>[6x]MNVQAHLFVSLGTAPAIVPEAFLLPGARFVSVHVLTTERPDVTLIREFFRRHAPGVNLTITRVAGFQDLKSEEDHFRFEEVMFRWFLASRTGPEQRFVCLTGGFKTMSAAMQKAATVLGAAEVFHVLADDCCVGPQGRLMPPSTLEEILWARDQGHLHWIRLGPERGWPQLRRIA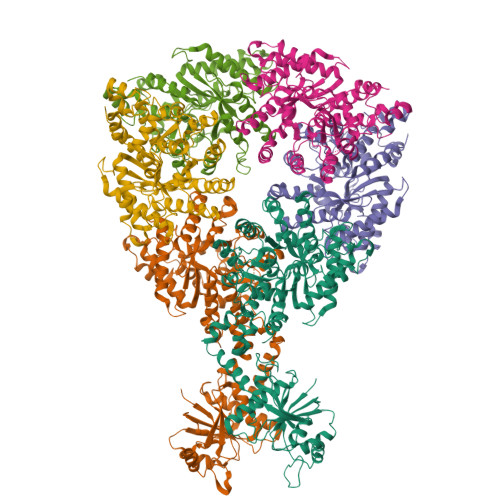PEQFPLQVVEEKGDERRVQAEDRAFGTFLQDLLQRASRIAGAWEMLPELPFADLATWSEGELAWLREPLDPRAPADQRWVAGLPKIELHCHLGGFATHGELLRRVRNAAENPGKLPPLEEPRLPEGWPLPAQPIPLAEYMKLGNANGTALLRDPGCLREQCRLLYRHLVDQGVCYAEVRCSPANYAEVRSPWDVLADIRAAFQECMEGARTAPGGLPACHVNLILIATRRASGDYRAAIARHLALAVTAAEHWRDENACRVVGVDLAGYEDEKTRAHYFREEFTAVHRCGLAVTVHAGENDDAEGIWRAVFDLNARRLGHALSLGQSRELLRSVADRGIGVELCPYANLQIKGFRLDGSDRAGPADPRHEAHAPGPYPLLDYLREGVRVTVNTDNIGISAASLTDNLLLAARLCPGLTRLDLLHLQRHALETAFCTATQRLTLLRRISSGIPRPHHHHHH>[8x]MGAGAGARWGSRAPEAPQPARAAGPGDVVVPCHGEHQAGIVTPPPSFIALVALDLASTSDRASVERLLRVWTVDIERLTTGRPGLADSEPELALVPAALTVTVGFGPGLLTAAGLRHRAPAWLHPLPP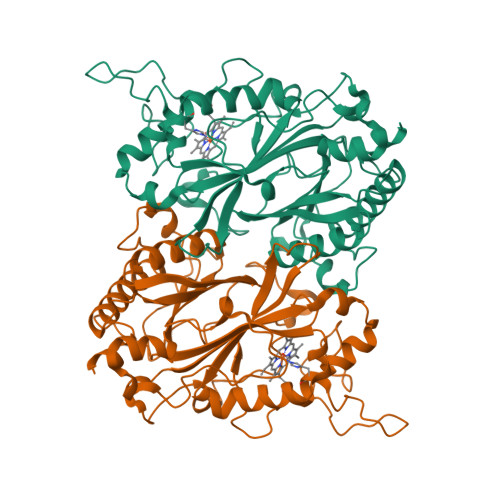FGIDRLDPAWCDGDVVLQVCADDRTTLAHAVRVLTKEAQGLASVRWVQRGFRRSPGISEPDGTSMRNLMGQVEGTANLDPRTDPDLLWHRDGEPGWLTGGTSMVVRRIAMNLDTWDELSRGAREATIGRTLRTGAPLTGRAEHDEPDLEALDDHGRPVIDLEAHIRRARPTQREETFLRRAYNYDEAPPPGRASDSGLLFVTYQRDVDAQFTPVQRRLDAADLLNEWTFPVGSAVFAVPGGWSAGEYVGQRLLEG> MSTVKAPTLPASIFRAYDIRGVVGDTLTAETAYWIGRAIGSESLARGEPC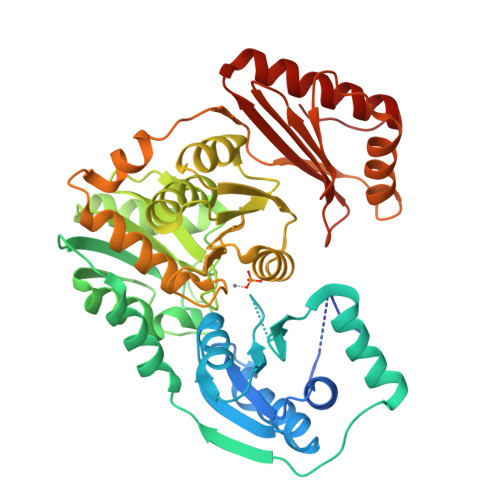VAVGRDGRLSGPELVKQLIQGLVDCGCQVSDVGMVPTPVLYYAANVLEGKSGVMLTGCHNPPDYNGFKIVVAGETLANEQIQALRERIEKNDLASGVGSVEQVDILPRYFKQIRDDIAMAKPMKVVVDCGNGVAGVIAPQLIEALGCSVIPLYCEVDGNFPNHHPDPGKPENLKDLIAKVKAENADLGLAFDGDGDRVGVVTNTGTIIYPDRLLMLFAKDVVSRNPGADIIFDVKCTRRLIALISGYGGRPVMWKTGHSLIKKKMKETGALLAGEMSGHVFFKERWFGFDDGIYSAARLLEILSQDQRDSEHVFSAFPSDISTPEINITVTEDSKFAIIEALQRDAQWGEGNITTLDGVRVDYPKGWGLVRASNTTPVLVLRFEADTEEELERIKTVFRNQLKAVDSSLPVPF>[2x]GSEAAQLLEAADFAARKHRQQRRKDPEGTPYINHPIGVARILTHEAGITDIVVLQAALLHDTVEDTDTTLDEVELHFGAQVRRLVEEVTDDKTLP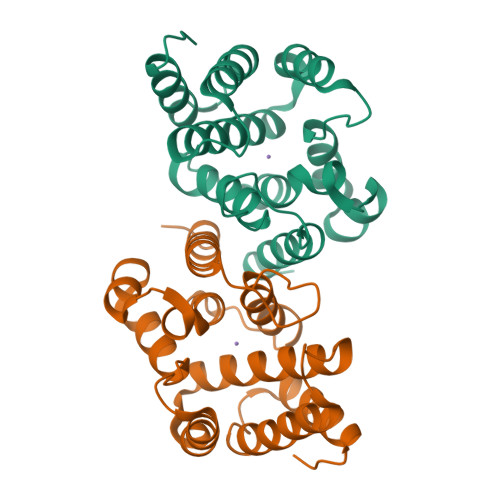KLERKRLQVEQAPHSSPGAKLVKLADKLYNLRDLNRCTPEGWSEHRVQEYFEWAAQVVKGLQGTNRQLEEALKHLFKQRGLTI> GPRSQTQPVPRFDETSTDTGGPIKIIDPEKVSKEPDALLEGFEWATLDLTNE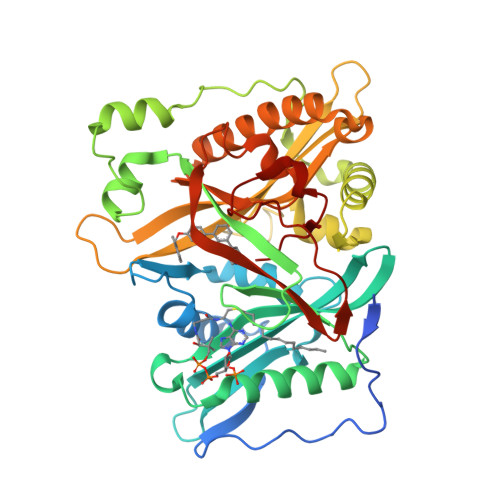TELQELWDLLTYHYVEDDNAMFRFRYSQSFLHWALMSPGWKKEWHVGVRATKSRKLVASICGVPTEINVRNQKLKVVEINFLCIHKKLRSKRLTPVLIKEITRRCYLNGIYQAIYTAGVVLPTPVSSCRYYHRPLDWLKLYEVGFSPLPAGSTKARQITKNHLPSTTSTPGLRPMEPKDIDTVHDLLQRYLSRFALNQAFTREEVDHWLVHKPETVKEQVVWAYVVEDPETHKITDFFSFYNLESTVIQNPKHDNVRAAYLYYYATETAFTNNMKALKERLLMLMNDALILAKKAHFDVFNALTLHDNPLFLEQLKFGAGDGQLHFYLYNYRTAPVPGGVNEKNLPDEKRMGGVGIVML> GDVQNAVEGAMVRVADTVQTSATNSERVPNLTAVETGHTSQAVPGDTMQTRHVINNHVRSESTIENFLARSACVFYLEYKTGTKEDSNSFNNWVITTRRVAQLRRKLEMFTYLRFDMEITVVITSSQDQSTSQNQNAPVLTHQIMYVPPGGPIPVSVDDYSWQTSTNPSIFWTEGNA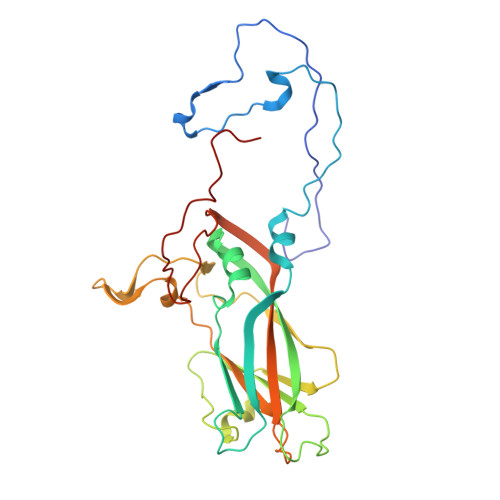PARMSIPFISIGNAYSNFYDGWSHFSQAGVYGFTTLNNMGQLFFRHVNKPNPAAITSVARIYFKPKHVRAWVPRPPRLCPYINSTNVNFEPKPVTEVRTNIITT> MHHHHHHHDGTENPIHDRTSDYHKYLKVKQGDSDLFKLTVSDKRYIWYNPDPKERDSYECGEIVSETSDSFTFKTVDGQDRQVKKDDAN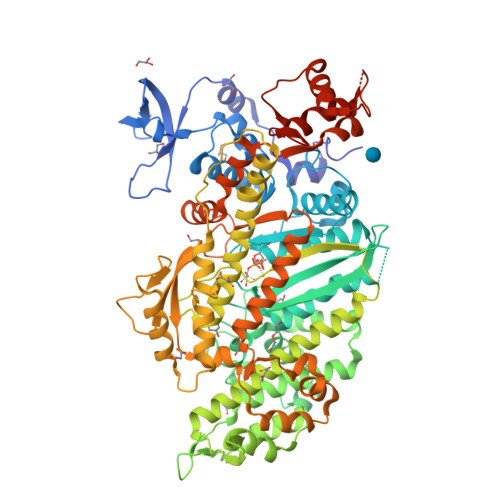QRNPIKFDGVEDMSELSYLNEPAVFHNLRVRYNQDLIYTYSGLFLVAVNPFKRIPIYTQEMVDIFKGRRRNEVAPHIFAISDVAYRSMLDDRQNQSLLITGESGAGKTENTKKVIQYLASVAGRNQANGSGVLEQQILQANPILEAFGNAKTTRNNNSSRFGKFIEIQFNSAGFISGASIQSYLLEKSRVVFQSETERNYHIFYQLLAGATAEEKKALHLAGPESFNYLNQSGCVDIKGVSDSEEFKITRQAMDIVGFSQEEQMSIFKIIAGILHLGNIKFEKGAGEGAVLKDKTALNAASTVFGVNPSVLEKALMEPRILAGRDLVAQHLNVEKSSSSRDALVKALYGRLFLWLVKKINNVLCQERKAYFIGVLDISGFEIFKVNSFEQLCINYTNEKLQQFFNHHMFKLEQEEYLKEKINWTFIDFGLDSQATIDLIDGRQPPGILALLDEQSVFPNATDNTLITKLHSHFSKKNAKYEEPRFSKTEFGVTHYAGQVMYEIQDWLEKNKDPLQQDLELCFKDSSDNVVTKLFNDPNIASRAKKGANFITVAAQYKEQLASLMATLEGGGNPHFVRCIIPNNKQLPAKLEDKVVLDQLRCNGVLEGIRITRKGFPNRIIYADFVKRYYLLAPNVPRDAEDSQKATDAVLKHLNIDPEQYRFGITKIFFRAGQLARIEEAREQRLESNEPPMDFDDDIPF> RCELKLIASPGSWRLYSARKID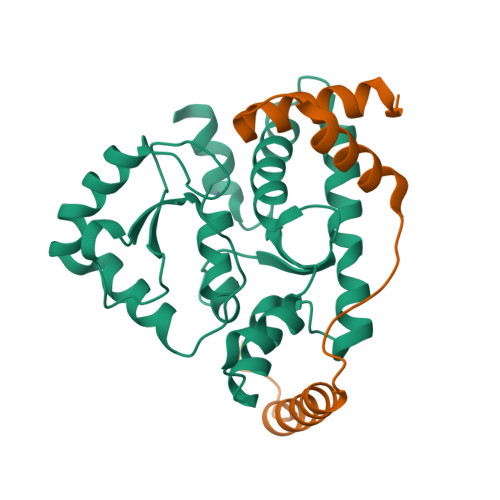ARFKSYEQKIFQRDRYTCQFCGFQAALYQDIVNLDGDYTNNRLSNLVTACCFCAQCFFVESVGVGGYGGGTLIYLPELTQAELNSLCHVLFCAITNDTGYKSSAQNIYRSFKFRSQIVEEKFGEGTSDPAIFGQLMIDSGVNSEEIREKLFKNIRLLPSRAKFRKQIEKWAAA;>[2x]VEPPPDDYLMKLQKQLASFQSILESGDLSINKAVENEEITLISKALKESTIVEPIERGVAALIAFHGQNE;> NVNQTMADNQQRCELKLIASPGSWRLYSARKIDERFKSYEQKIFQRDRYTCQFCGFQARLYQDIVNLDGDYTNNRLSNLVTACCFCAQCFFVESVGVGGYGGGTLIYLPELTQAELNSLCHVLFCAITNDTGYKSSAQNIYRSFKFRSQIVEEKFGEGTSDPAIFGQLMIDSGVNSEEIREKLFKNIRLLPSRAKFRKQIEKWAASALEEIAD> MVSCGGGRSVKNAACCAWFPVLDDIQANLFNGGKCEEEAHEAVRLTFHDAVGFSLAAQKAGKFGGGGADGSILAFSDIETAFIPNFGLEFTTEGFIPFALAHGVSFGDFVQFAGAVGAANCAGGPRLQFLAGR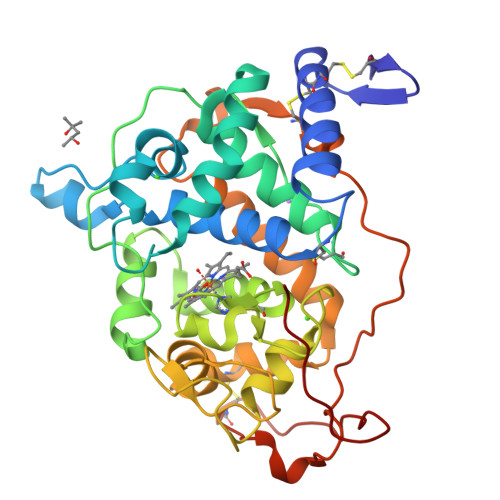SNISQPSPDGLVPDPTDSADKILARMADIGFSPTEVVHLLASHSIAAQYEVDTDVAGSPFDSTPSVFDTQFFVESLLHGTQFTGSGQGGEVMSPIPGEFRLQSDFALSRDPRTACEWQALVNNQQAMVNNFEAVMSRLAVIGQIPSELVDCSDVIPTPPLAKVAQVGSLPPGKSMADVQVACTNGMPFPSLPTSPGPVQTVAPVL>[6x]MARV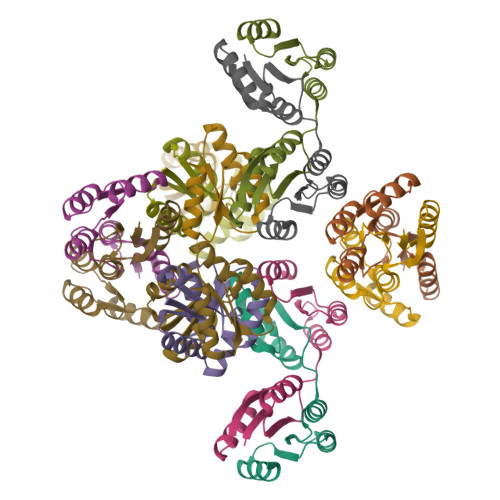LVVDDAAFMRMLLKKILTQAGHEVVGEASNGKEAVEKYKQLKPDLVTMDIVMPEMDGITAVKEIMKIDPNAKIIMITAVGQEAKVMEALKSGAKGYIVKPFQAQKVIEEVNRVLSS(2R)-2-(dihydroxymethyl)-2-hydroxy-3-oxobutyl dihydrogen phosphate | C5 H11 O8 P | 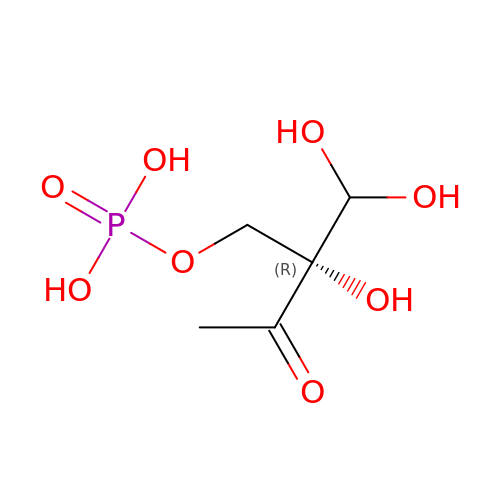IYNPDRWOJYWTNN-YFKPBYRVSA-N> MAPSARYESSSSDASALGKPLKFEFSGQSAPNRFLKGAMTERMSSWDPENLEARGVPSKNLINLYRRWGEGGIGLILTGNIMIEYDQLEAAGNPIIPRDSDFSGERFEAFKELATEAKKHGSL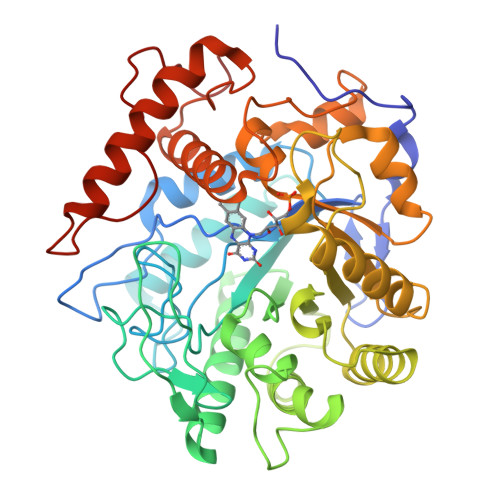IVGQVSHPGRQVESKIQKNPVSASDVQLKGEVMGMTFAKPRAATDEDIANIIQGFVHAAQYLEKAGYSGIELHGAHGYLLAQFLSPTTNKRTDKYGGSIENRARIIVEITDAIRKRVSSSFVVGIKLNSVEFQDNGFNPDEARQICKILEENKFDFVELSGGTYEKNAFVHQRETTKKREGFFLEFAESIAPVLSKTKTYITGGFKSVGAMVAALDVVDGVGLARPLAQEPRLCKDILEGTVTGAIKQRIDENNFILTNIAAGTQMRLVGKDQEPIDLSQEENMGPFLQDVGTWTEKMANNTNQREYGYVDITSAQVVPYGTASG>[2x]MSTLKVVSSKLAAEIDKELMGPQIGFTLQQLMELAGFSVAQAVCRQFPLRGKTETEKGKHVFVIAGPGNNGGDGLVCARHLKLFGYNPVVFYPKRSE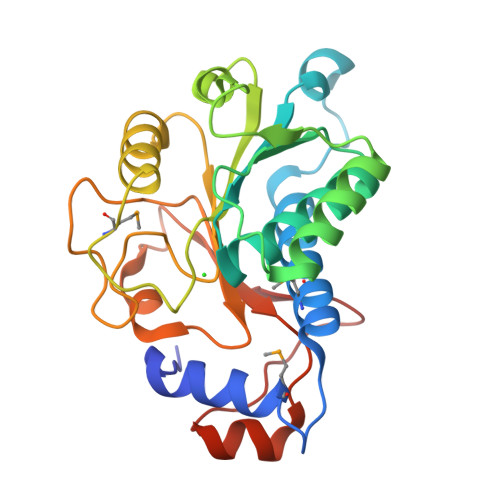RTEFYKQLVHQLNFFKVPVLSQDEGNWLEYLKPEKTLCIVDAIFGFSFKPPMREPFKGIVEELCKVQNIIPIVSVDVPTGWDVDKGPISQPSINPAVLVSLTVPKPCSSHIRENQTTHYVGGRFIPRDFANKFGFEPFGYESTDQILKL>SNAMNALAATNRNFKLAARLLGLDSKLEKSLLIPFREIKVECTIPKDDGTLASFVGFRVQHDNARGPMKGGIRYHPEVDPDEVNALAQLMTWKTAVAKIPYGGAKGGIGCDPSKLSISELERLTRVFTQKIHDLIGIHTDVPAPDMGTGPQTMAWILDEYSKFHGYSPAVVTGKPIDLGGSLGRDAATGRGVMFGTEALLNEHGKTISGQRFVIQGFGNVGSWAAKLISEKGGKIVAVSDITGAIKNKDGIDIPALLKHTKEHRGVKGFDGADPIDPNSILVEDCDILVPAALGGVINRENANEIKAKFIIEAANHPTDPDADEILSKKGVVILPDIYANSGGVTVSYFEWVQNIQGFMWEEEKVNDELKTYMTRSFKDLKEMCKTHSCDLRMGAFTLGVNRVAQATILRGWGA[6x]

GDHs release the ammonium cation from glutamate in a reversible, NAD(P)+-dependent oxidative deamination reaction that yields 2OG. We have provided detailed structural and kinetic information about the functioning of AtGDH1, one of three mitochondrial NAD+-dependent GDHs in A. thaliana. The asymmetric unit of both crystal structures is comprised of a homohexameric oligomer with non-crystallographic 32 (D3) symmetry. A subunit of AtGDH1 is comprised of 411 amino acid residues (44.5 kDa) and can be subdivided into two domains.

In our apo-structure, all subunits are in the open conformation, even though the position of domain II varies by as much as 11.3°, with χ between 62.0° and 73.3°. Comparison of AtGDH1-apo and the NAD+ complex shows only minor rearrangements within the coenzyme binding site, which suggests that apo AtGDH1 is already well prepared to accept the coenzyme. The homohexameric assembly is in agreement with the size-exclusion elution profile (not shown), as well as with analysis of inter-subunit contacts by PISA (Protein Interfaces, Surfaces and Assemblies), which estimated the surface area buried upon hexamer formation at 23220 Å2 and the total surface area at 87480 Å2 (for AtGDH1-apo structure). What is unique about AtGDH1 and has never been observed in any GDH structure, is binding of a potassium cation, seen in both structures of AtGDH1 presented in this work, as confirmed by the CheckMyMetal server. The residues involved in potassium coordination are Ser27, Ile30, and Glu38∗ (from another subunit).> QRFPQRYIELAIVVDHGMYKKYNQNSDKIKVRVHQMVNHINEMYRPLNIAISLNRLQIWSKKDLITVKSASNVTLESFGNWRETVLLKQQNNDCAHLLTATNLNDNTIGLAYKKGMCNPKLSVGLVQDYSPNVFMVAVTMTHELGHNLGMEHDDKDKCKCEACIMSDVISDKPSKLFSDCSKNDYQTFLTKY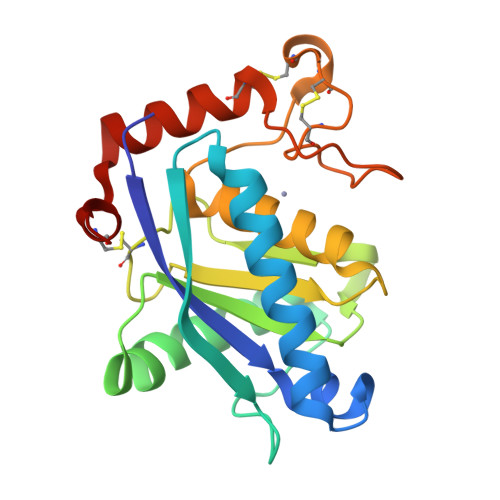NPQCILNAP>MARMGDFGVVDYTSLMALAPRSKNFLELLGVFSESNTRYIDSRYAEFEREEKGVTKMNAMARGGSRKYIGSEKARKEIIEVPFAPLDGVTVASEV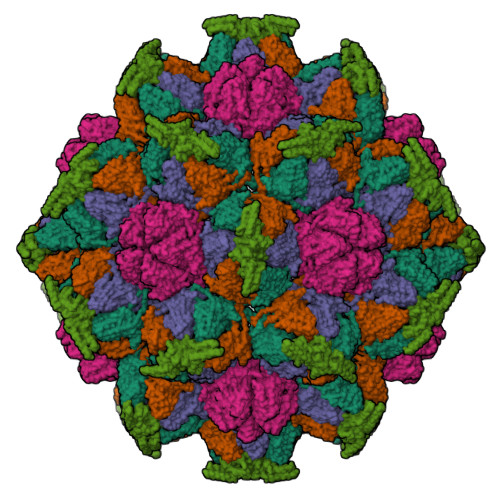EAFRQYGTESQTASVEALVQRKIEHIQRSHGIYIRDCQYTALLKDKILAEDEDGNEITALAKNFSTLWGVSRKTGAINTTTAVNPFSVLATKRQEIIDSMGENNGFTSMVVLCTTRDFNAIVDHPDVRAAYEGRDGGAEYLTRRLGDAVDFQVFTHKGVTLVEDTSGKLTDGSAYMFPLGVQDMFQAVYAPADSTDHVNTISQGSYLFLNAGENWRRDVIESEVSYACMVTRSELICDLTITVAHHHHHH[4x];> MTTITTTTNNTFDLANVIAEYKAGFEQYKADNKQYNADAYRRKIESINSDAALTNGAFNQFAYGSQMFEGKTLQEIAESLKTMQVKDSSREDENGLIFPHVTLQLVSPTTPAQYYGLIAEAVKLGFEVCPDWRLHVGTGRNFPACRLVRQAEWYKPHNEKLMAERIAEAEKQEAERLKAEYFNEHRVQAYVEQAQRKFMATQAQQAAISLSAAISRELYASSGLSDDDLAVVAQSDVWAFNTLAPQLQEKDPNVISAALTGAGFVKGKHKLSDGKQATLWVKDGADVTALTLESKYIQ> MFLKRLDVIGFKSFAERISVDFVKGVTAVVGPNGSGKSNITDAIRWVLGEQSARSLRGGKMEDI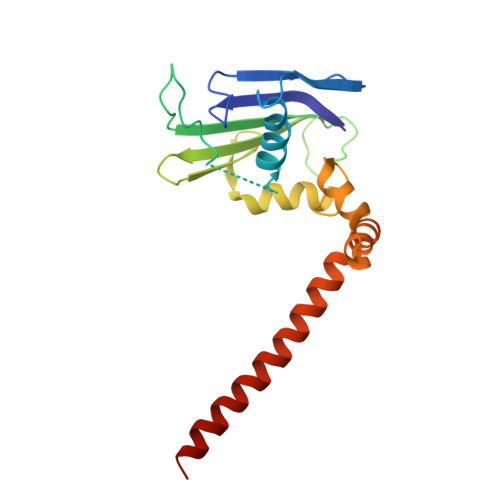IFAGSDSRKRLNLAEVTLTLDNDDHFLPIDFHEVSVTRRVYRSGESEFLINNQPCRLKDIIDLFMDSGLGKEAFSIISQGKVEEILSSKAEDRRSIFEEAAGVLKYKTRKKKAENKLFETQDNLNRVEDILHELE(2R,3Z,5R)-3-(2-HYDROXYETHYLIDENE)-7-OXO-4-OXA-1-AZABICYCLO[3.2.0]HEPTANE-2-CARBOXYLIC ACID | C8 H9 N O5 | 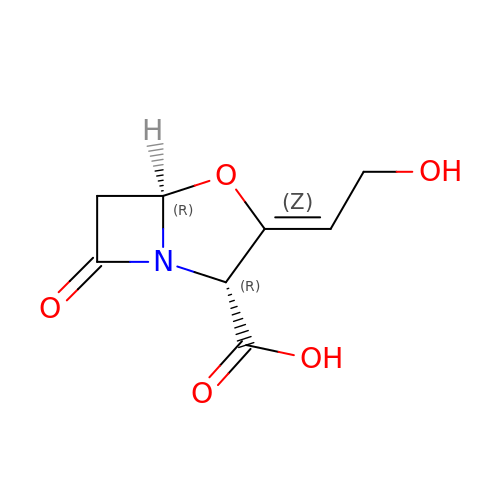HZZVJAQRINQKSD-PBFISZAISA-N>MAEELVLERCDLELETNGRDHHTADLCREKLVVRRGQPFWLTLHFEGRNYEASVDSLTFSVVTGPAPSQEAGTKARFPLRDAVEEGDWTATVVDQQDCTLSLQLTTPANAPIGLYRLSLEASTGYQGSSFVLGHFILLFNAWCPADAVYLDSEEERQEYVLTQQGFIYQGSAKFIKNIPWNFGQFEDGILDICLILLDVNPKFLKNAGRDCSRRSSPVYVGRVGSGMVNCNDDQGVLLGRWDNNYGDGVSPMSWIGSVDILRRWKNHGCQRVKYGQCWVFAAVACTVLRCLGIPTRVVTNYNSAHDQNSNLLIEYFRNEFGEIQGDKSEMIWNFHCWVESWMTRPDLQPGYEGWQALDPTPQEKSEGTYCCGPVPVRAIKEGDLSTKYDAPFVFAEVNADVVDWIQQDDGSVHKSINRSLIVGLKISTKSVGRDEREDITHTYKYPEGSSEEREAFTRANHLNKLAEKEETGMAMRIRVGQSMNMGSDFDVFAHITNNTAEEYVCRLLLCARTVSYNGILGPECGTKYLLNLNLEPFSEKSVPLCILYEKYRDCLTESNLIKVRALLVEPVINSYLLAERDLYLENPEIKIRILGE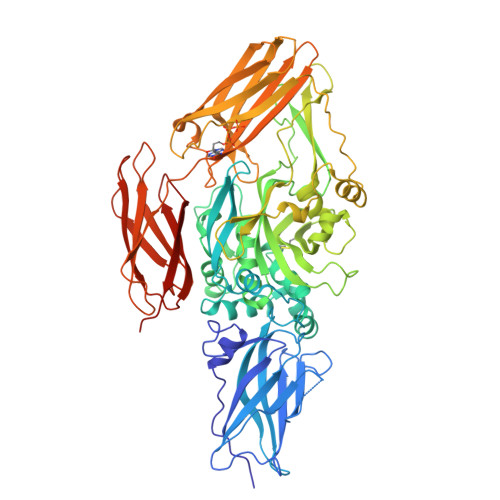PKQKRKLVAEVSLQNPLPVALEGCTFTVEGAGLTEEQKTVEIPDPVEAGEEVKVRMDLLPLHMGLHKLVVNFESDKLKAVKGFRNVIIGPALEHHHHHHHH[3x]>STNDNIKDLLDWYSSGSDTFTNSEVLDNSLGSMRIKNTDGSISLIIFPSPYYSPAFTKGEKVDLNTKRTKKSQHTSEGTYIHFQISGVTNTEKLPTPIELPLKVKVHGKDSPLKYWPKFDKKQLAISTLDFEIRHQLTQIHGLYRSSDKTGGYWKITMNDGSTYQSDLSKKFEYNTEKPPINIDEIKTIEA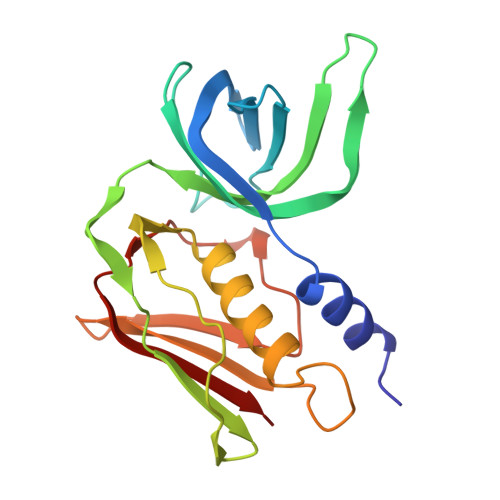EIN[3x]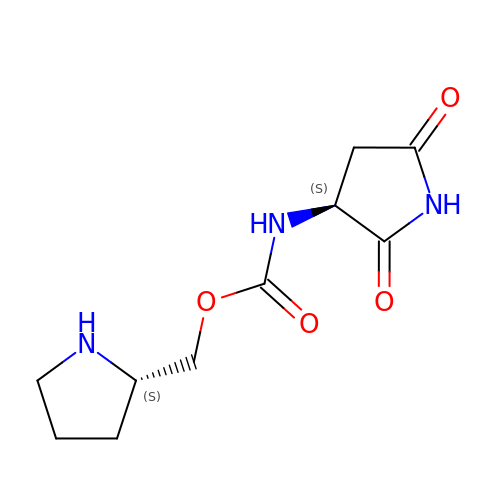[(2~{S})-pyrrolidin-2-yl]methyl ~{N}-[(3~{S})-2,5-bis(oxidanylidene)pyrrolidin-3-yl]carbamate | C10 H15 N3 O4 | BROVZDKFOULGAP-BQBZGAKWSA-N> WGNLGHETVAYIAQSFVASSTESFCQNILGDDSTSYLANVATWADTYKYTDAGEFSKPYHFIDAQDNPPQSCGVDYDRDCGSAGCSISAIQNYTNILLESPNGSEALNALKFVVHIIGDIHQPLHDENLEAGGNGIDVTYDGETTNLHHIWDTNMPEEAAGGYSLSVAKTYADLLTERIKTGTY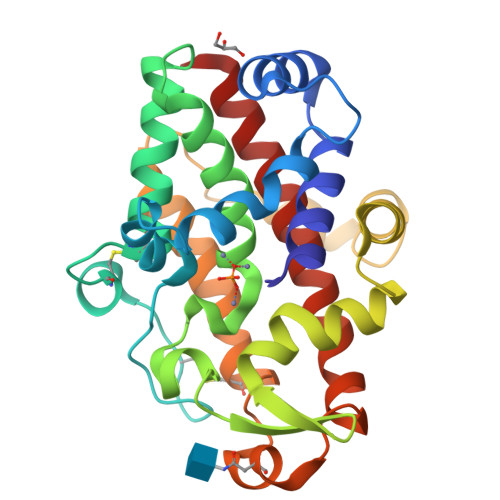SSKKDSWTDGIDIKDPVSTSMIWAADANTYVCSTVLDDGLAYINSTDLSGEYYDKSQPVFEELIAKAGYRLAAWLDLIASQPS>[2x]MGRGSHHHHHHGMAMNIKELSLHELCEELKTPAWNVPLTFVGDVGGTSARMGFVREGKNDSVHACVTRYSMKRKDITELIEFFNEIIELMPASVIKRVKAGVINVPGPVTGGAVGGPFNNLKGIARLSDYPKALFPPGRSAILNDLEAGGFGVLAVSDAHVFSEYFGVMWEGTQWRTCEQEPAGSV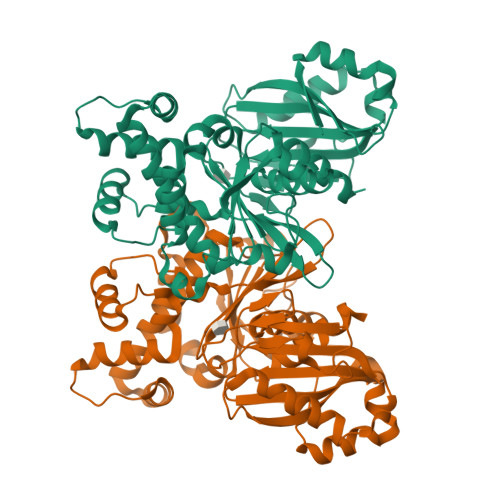IGRGRCLVLAPGTGLGSSLIYYNPMNQQHIVVPLELGSQTIPMRKDIDYIQTLHAELKLLPNYENMVSGAGLEFHYRQVVRGSRPPCSAGEIAKLASEGDANACKAMKKYHEYLMRVGSEASMALLPLTIVLVGDNIVNNAFFYRNPQNLKEMHREALNHEMERFGFQSRVTYLRQKKLLNLNLMGCYRCGLDLS>[2x]LGSMKTERWVVREHVEGVPDAARIYEKVETELNTRLGEEQMLLKTLYVSVDPYLQGICLDTPIGDHMGADSIMQVLDAGPNAPFRPGDLVQGFGGWRTHLVSDGKPKLWQTGTFPMVFPAYRKLDLRHYDDALPLSTALGVMGGPGMTAWGTMTKFM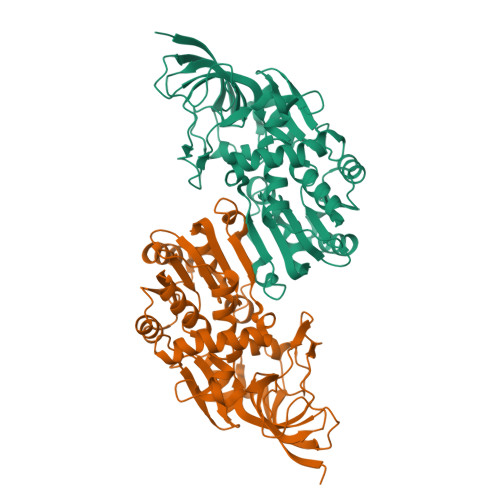QVRPGDTVVVSGASGMIGTLVGQMAKRAGARVVGTAGSAGKARYLSQLGFDAVIDYKLADDADKMREALREAAPDGVDKYFDSIGGSVTDAVFSMLNVGSQVAVCWQWATQVQRDYHGPRLLPYIMFPRATIRGIFSLEWFTEQNWSALHEELGGLVRRQELVAHETVQDGFEHIPAAYQTLFSASESNRGKVLVRV> MTSRDQPRPKGPPKSTSPCPGISNSESSPTLNYQGILNRLKQFPRFSPHFAAELESIYYSLHKIQQDVAEHHKQIGNVLQIVESCSQLQGFQSEEVSPAEPASPGTPQQVKDKTLQESSFEDIMATRSSDWLRRPLGEDNQPETQLFWDKEPWFWHDTLTEQLWRIFAGVHDEKAKPRDRQQAPGLGQESKAPGSCDPGTDPCPEDASTPRPP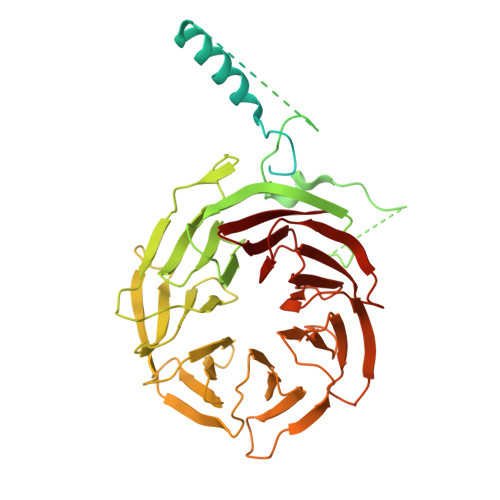EASSSPPEGSQDRNTSWGVVQEPPGRASRFLQSISWDPEDFEDAWKRPDALPGQSKRLAVPCKLEKMRILAHGELVLATAISSFTRHVFTCGRRGIKVWSLTGQVAEDRFPESHLPIQTPGAFLRTCLLSSNSRSLLTGGYNLASVSVWDLAAPSLHVKEQLPCAGLNCQALDANLDANLAFASFTSGVVRIWDLRDQSVVRDLKGYPDGVKSIVVKGYNIWTGGPDACLRCWDQRTIMKPLEYQFKSQIMSLSHSPQEDWVLLGMANGQQWLQSTSGSQRHMVGQKDSVILSVKFSPFGQWWASVGMDDFLGVYSMPAGTKVFEVPEMSPVTCCDVSSNNRLVVTGSGEHASVYQITY2',3'-DIDEOXY-THYMIDINE-5'-TRIPHOSPHATE | C10 H17 N2 O13 P3 | 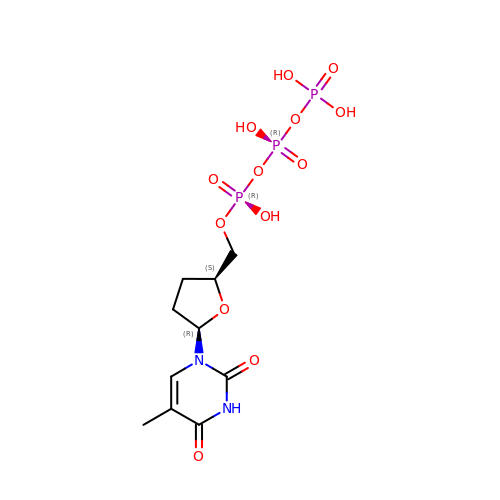URGJWIFLBWJRMF-JGVFFNPUSA-N>[4x]XSLSSKQKATVKDFFSKMSTRSDDIGAEALSRLVAVYPQTKSYFSHWKDASPGS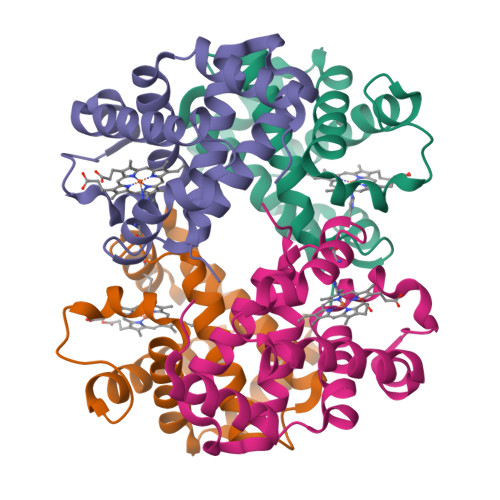APVRKHGITIMGGVYDAVGKIDDLKGGLLSLSELHAFMLRVDPVNFKLLAHCMLVCMSMIFPEEFTPQVHVAVDKFLAQLALALAEKYR;>VEWTDSERAIITSIFSNLDYEEIGRKSLCRCLIVYPWTQRYFGAFGNLYNAETILANPLIAAHGTKILHGLDRALKNMDDIKNTYAELSLLHSDKLHVDPDNFRLLADCLTVVIAAKMGSAFTVDTQVAWQKFLSVVVSALGRQY[4x]> GSPGISGGGGGSQNSLALHKVIMVGSGGVGKSALTLQFMYDEFVEDYEPTKADSYRKKVVLDGEEVQIDILDTAGQEDYAAIRDNYFRSGEGFLCVFSITEMESFAATADFREQILRVKEDENVPFLLVGNKSDLEDKRQVSVEEAKNRAEQWNVNYVETSAKTRANVDKVFFDLMREIRARKMEDS;> GSPGISGGGGGSAYSNTYQEFTNIDQAKAWGNAQYKKYGLSKSEKEAIVSYTKSASEINGKLRQNKGVINGFPSNLIKQVELLDKSFNKMKTPENIMLFRGDDPAYLGTEFQNTLLNSNGTINKTAFEKAKAKFLNKDRLEYGYISTSLMNVSQFAGR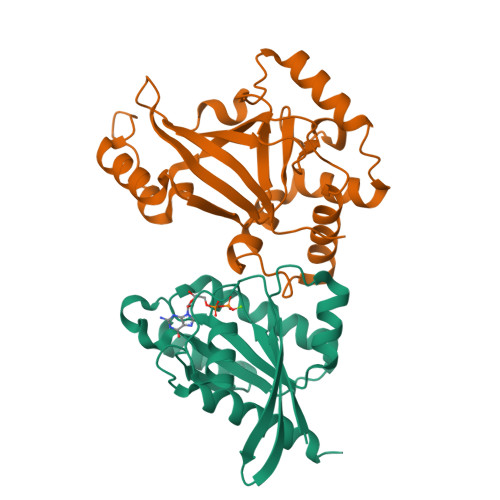PIITKFKVAKGSKAGYIDPISAFAGQLEMLLPRHSTYHIDDMRLSSDGKQIIITATMMGTAINPK>MALDNLLRHLKISKEQ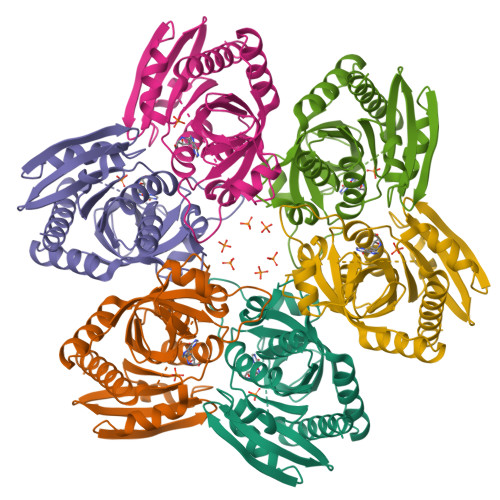ITPVVLVVGDPGRVDKIKVVCDSYVDLAYNREYKSVECHYKGQKFLCVSHGIGSAGCAICFEELCQNGAKVIIRAGSCGSLQPDLIKRGDICICNAAVREDRVSHLLIHGDFPAVGDFDVYDTLNKCAQELNVPVFNGISVSSDMFYPNKIIPSRLEDYSKANAAVVEMELATLMVIGTLRKVKTGGILIVDGCPFKWDEGDFDNNLVPHQLENMIKIALGACAKLATKYAKGEFEAYVEQKLISEEDLNSAVDHHHHHH[2x]> GHMSESREARLIIFHAGSLSIPLSQVEEKFTKYAQEKLGVKVTFQDEASGSVKAVRKVTDLKKRADIVAVADYTLIPQLMIPNYTDFYVLFATNEIVIAFTNKSKYADEMLKNPDKWYEILSRPDVSFGFSDPNQDPCGYRSVMVMKLAELYYGRP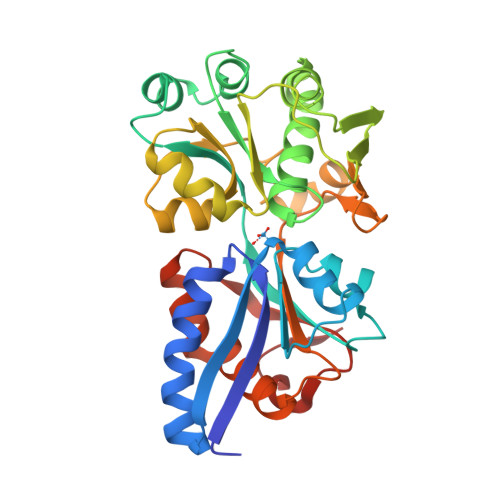IFKELVEKTTNIYSNGTRIYAPKEIIIKDKRVIMRPKETDLVGLVESGSLDYIFIYKSVAKQHHLSYITLPDDINLGDFNKADFYGRVSITLGSTGKTIKAKPIVYGITVLKNAPNRELAIEFLRFLLGNEGRKIFEDNYQEFLSPPVAFGNVPPEIRRLVEVK5'-O-[(R)-(carboxyoxy)(hydroxy)phosphoryl]adenosine | C11 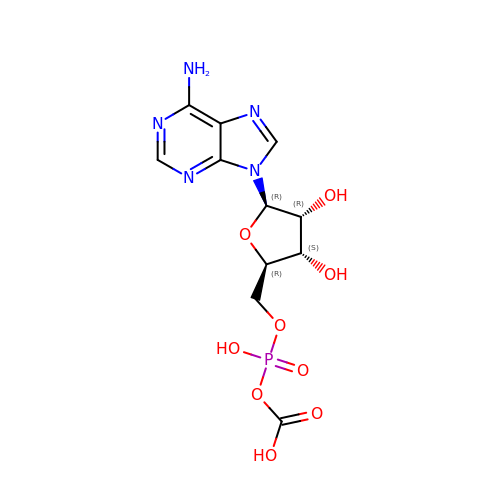H14 N5 O9 P | ZYLWEGVHTNBJTI-KQYNXXCUSA-N(6R,6aS,10S,10aR)-10-methyl-4-phenyl-6-[(1E)-prop-1-en-1-yl]-2,6,6a,7,8,9,10,10a-octahydro-1H-[2]benzopyrano[4,3-c]pyridin-1-one 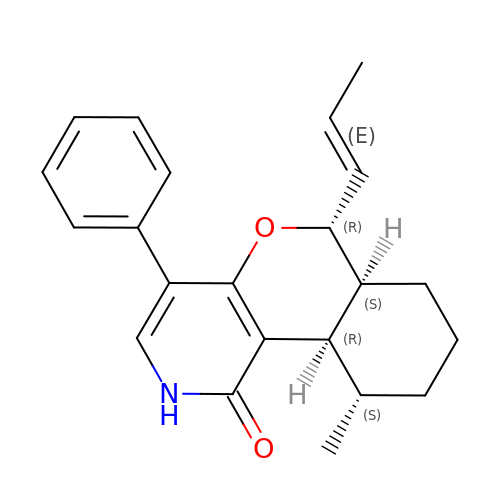| C22 H25 N O2 | ZBTREMSWPKVXFU-GQECYKNHSA-N N-(4-{[3-(trifluoromethyl)phenyl]sulfonyl}benzyl)-2H-pyrazolo[3,4-b]pyridine-5-carboxamide 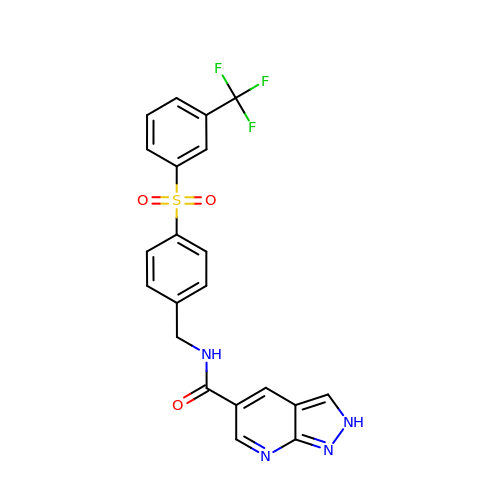| C21 H15 F3 N4 O3 S | LKBHAGGICJWHQQ-UHFFFAOYSA-N> HPYYLRSFLVVLKTVLENEDDMLLFDEQEKGIVTKFYQLSATGQKLYVRLFQRKLSWIKMTKLEYEEIALDLTPVIEELTNAGFLQTESELQELSEVLELLSAPELKSLAKTFHLVNPNGQKQQLVDAFLKLAKQRSVCTWGKNKPGIGAVILKRAKALAGQSVRICKGPRAVFSRILLLFSLTDSMEDEDAACGGQGQLSTVLLVNLGRMEFPSYTINRKTHIFQDRDDLIRYAAATHMLSDISSAMANGNWEEAKELAQCAKRDWNRLKNHPSLRCHEDLPLFLRCFTVGWIYTRILSRFVEILQRLHMYEEAVRELESLLSQRIYCPDSRGRWWDRLALNLHQHLKRLEPTIKCITEGLADPEVRTGHRLSLYQRAVRLRESPSCKKFKHLFQQLPEMAVQDVKHVTITGRLCPQRGMCKSVFVMEAGEAADPTTVLCSVEELALAHYRRSGFDQGIHGEGSTFSTLYGLLLWDIIFMDGIPDVFRNACQAFPLDLCTDSFFTSRRPALEARLQLIHDAPEESLRAWVAATWHEQEGRVASLVSWDRFTSLQQAQDLVSCLGGPVLSGVCRHLAADFRHCRGGLP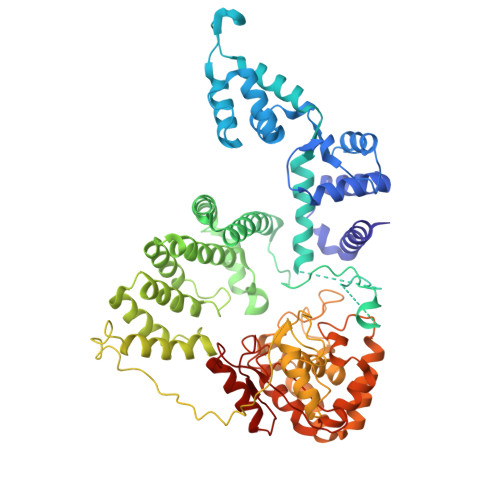DLVVWNSQSRHFKLVEVKGPNDRLSHKQMIWLAELQKLGAEVEVCHVVAVG>[5x]MGRAHKETLDKLTNAAINKINLLNTSKVKYLVSSAFAGLYVGIGILLIFTIGGLLTDAGSPMTKIVMGLSFAIALSLVIMTGTELFTGNNMVMSAGMLNKGVSIKDTS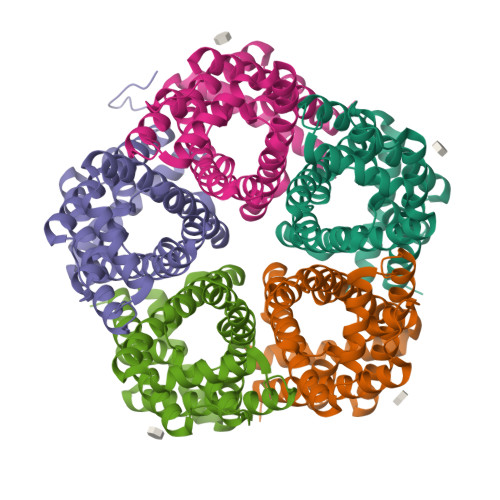KIWAYSWVGNLIGALVLGIIFVGTGLVDKGPVAEFFANTAASEASMPFTALFFRGILCNILVCVSVLCSFRTNSDTAKIIMIFLCLFAFITSGFEHSVANMTIYSVSLFSPTISTVTIGGAIYNLVAVTLGNIVGGALFMGLGTYILGKEKLNAAAENLY TIM family proteins exhibit a classical type I membrane protein structure with an N-terminal immunoglobulin variable Ig-like (Ig V) domain, a heavily O-linked-glycosylated mucin-like domain (MLD) and a short C-terminal cytoplasmic tail. Recent studies indicate that hTIM-1, with some other but not all phosphatidylserine (PS) binding receptors, functions as a common attachment factor for a range of enveloped viruses, including filoviruses, flaviviruses, HIV, etc., through direct interaction with PS of the viral envelope. The Ig V domains of hTIM-1 and hTIM-4, exhibit two antiparallel β sheets with the front and back faces formed by A, G, F, C, C′, C″ and B, E, D strands respectively. A hydrophobic cleft formed by CC’ and FG loops, located at an equivalent position in hTIM-1 and hTIM-4 structures represents the putative PS ligand binding site.

We crystallized the Ig V domains of hTIM-1 and hTIM-4 and determined the structures at a resolution of 1.3 Å and 2.3 Å, respectively, using the molecular replacement method. While hTIM-1 has only one molecule in the asymmetric unit, there are eight molecules of essentially the same structure present in the asymmetric unit of hTIM-4. A striking structural observation that was confirmed by sequence analysis indicates that the Ig V domains of hTIM-1 and hTIM-4 share similarity with the N-terminal immunoglobulin-like domain of sialecsialo adhesin 1 (SnD1), hTIM-1 and hTIM-4 could be superimposed over the structure of SnD1 with an r.m.s. deviation of 2.3 Å and 2.2 Å, respectively. Residues known to interact with PS, including WFND of the FG loop, are conserved among hTIM-1, mTIM-1, hTIM-4 and mTIM-4. As to hTIM-4 and mTIM-4, three extra residues from the BC loop fill in the gap between the FG and BC loop. Results of binding assays performed using SPR showed that amongst the proteins tested only hTIM-1 Ig V could bind EBOV GP. A series of chimeras of hTIM-1 that binds EBOV GP and hTIM-4 that does not bind EBOV GP, where corresponding structural elements were exchanged, were generated to map the region(s) that are important for Ebola GP binding. As expected, the T14 (BC-CC’-FG) chimera showed the most dramatic loss in binding activity to GP, whilst the T41 (BC-CC’-FG) chimera restored the binding activity to GP. In agreement with hTIM-1 chimeras, the T41 (BC-CC’) and T41 (CC’-FG) chimeras gained some ability of binding to GP, but with a lower affinity of 73 and 208 μmol/L, respectively. Expression levels of hTIM-1, hTIM-4, mTIM-1 and mTIM-4 on the cell surface were close by transient transfection of the indicated amounts of a TIM-expressing plasmid, but hTIM-1 enhanced EBOV pseudovirus entry significantly greater than hTIM-4 and mTIM-4 (>3-fold when transfected with 0.5 μg).

>[8x]MVTSETVVTEVLGHRVTLPCLYSSWSHNSNSMCWGKDQCPYSGCKEALIRTDGMRVTSRKSAKYRLQGTIPRGDVSLTILNPSESDSGVYCCRIEVPGWFNDVKINVRLNLQRA>HHHGIRMTRISREMMKELLSVYFIMGSNNTKADPVTVVQKALKGGATLYQFREKGGDALTGEARIKFAEKAQAACREAGVPFIVNDDVELALNLKADGIHIGQEDANAKEVRAAIGDMILGVAAHTMSEVKQAEEDGADYV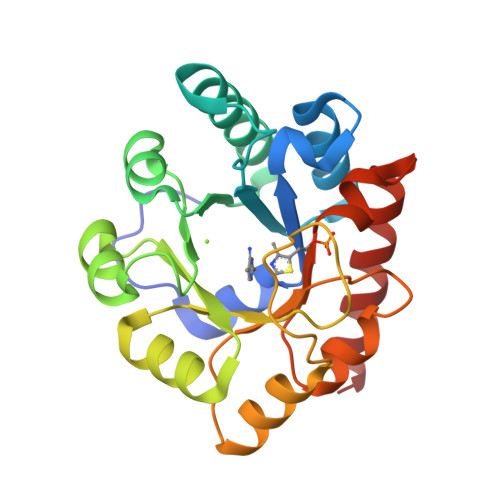GLGPIYPTETKKDTRAVQGVSLIEAVRRQGISIPIVGIGGITIDNAAPVIQAGADGVSMISAISQAEDPESAARKFREEIQTYKTGR[2x]>UUGCGUCACGCCGGCGA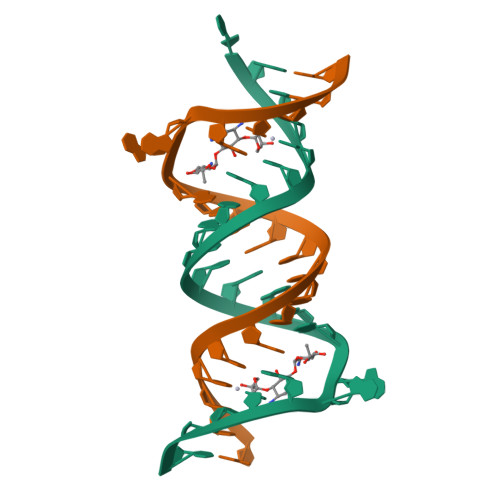AGUCGC[2x]> MDVVRASRNAKVKGKFRESYLSPAQSVKPKINTEEKLPREKLNPPTPSIYLESKRDAFSPVLLQFCTDPRNPITVIRGLAGSLRLNLGLFSTKTLVEASGEHTVEVRTQVQQPSDENWDLTGTRQIWPCESSRSHTTIAKYAQYQASSFQES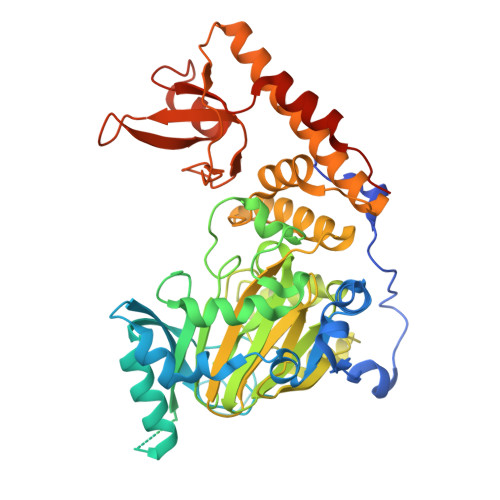LQEEKESEDEESEEPDSTTGTPPSSAPDPKNHHIIKFGTNIDLSDAKRWKPQLQELLKLPAFMRVTSTGNMLSHVGHTILGMNTVQLYMKVPGSRTPGHQENNNFCSVNINIGPGDCEWFAVHEHYWETISAFCDRHGVDYLTGSWWPILDDLYASNIPVYRFVQRPGDLVWINAGTVHWVQATGWCNNIAWNVGPLTAYQYQLALERYEWNEVKNVKSIVPMIHVSWNVARTVKISDPDLFKMIKFCLLQSMKHCQVQRESLVRAGKKIAYQGRVKDEPAYYCNECDVEVFNILFVTSENGSRNTYLVHCEGCARRRSAGLQGVVVLEQYRTEELAQAYDAFTLAPASTSRHHHHHH> GSAGQPLHETRPFLIKSGELTPGISALEYYERRIRLAETLPPKSCVILAGNDIQFASGAVFYPFQQEND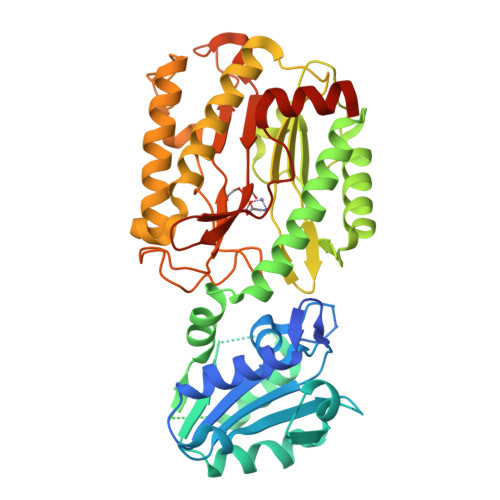LFYLSGWNEPNSVMILEKPTDSLSDTIFHMLVPPKDAFAEKWEGFRSGVYGVQEIFNADESASINDLSKYLPKIINRNDFIYFDMLSTSNPSSSNFKHIKSLLDGSGNSNRSLNSIANKTIKPISKRIAEFRKIKSPQELRIMRRAGQISGRSFNQAFAKRFRNERTLDSFLHYKFISGGCDKDAYIPVVATGSNSLCIHYTRNDDVMFDDEMVLVDAAGSLGGYCADISRTWPNSGKFTDAQRDLYEAVLNVQRDCIKLCKASNNYSLHDIHEKSITLMKQELKNLGIDKVSGWNVEKLYPHYIGHNLGLDVHDVPKVSRYEPLKVGQVITIEPGLYIPNEESFPSYFRNVGIRIEDDIAIGEDTYTNLTVEAVKEIDDLENVMQNGLSTKFEEDQVAPL>MASISEKMVEALNRQINAEIYSAYLYLSMASYFDSIGLKGFSNWMRVQWQEELMHAMKMFDFVSERGGRVKLYAVEEPPSEWDSPLAAFEHVYEHEVNVTKRIHELVEMAMQEKDFATYNFLQWYVAEQVEEEASALDIVEKLRLIGEDKRALLFLDK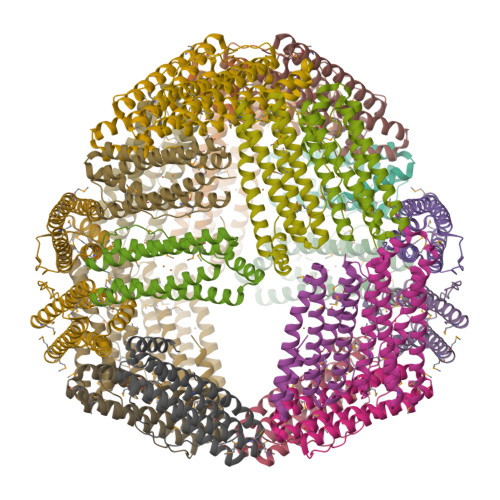ELSLRQFTPPAEEEK[12x]> HMQHITVRLPKKARAMIVGEITNVFKDKYPIADKLKVIPEYDVIEQDLCKLLSPGFPKQPLRVYKFGSRITGIGNRSSDLDLFVDIGNTFHTFEHRASNATVAKLRAMRKFFCDSEDWRLINFIEQARVPIIKTCHLPTGIECAICLNSMGFCNTNLLKYIFESQPLTQYMCIYVKNWLERCKLTEQISTYSITLMVIYFLQLQALLPPIAMLQIEDAANQAVLVGPWVVNFAQKSFSELGLQQLKATVPVIKGFLRNFFAYFAKFDYEHFLVCPYIGQANVEI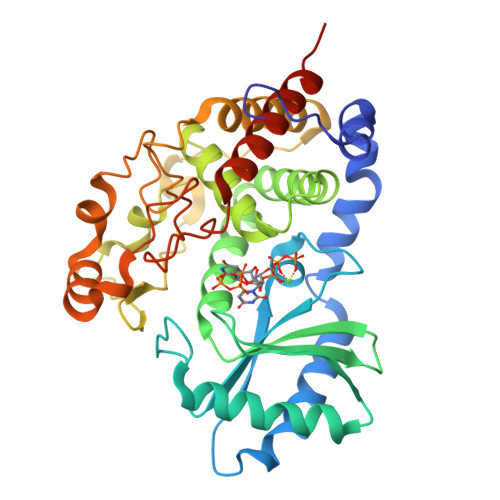AKIERMLHARYSAYVSDNPECSIQLKKPMVVQDPIQLNHNVTKAVTKYGLQTFVDYCQQTAELLEEPSTNWRQRYAF>[2x]MKELFQKIWQNELQFLNFDAKFQDKSKLDTAECAIILSVNKDNYERYFLLKEFQELCKKIDLRVDIFSMQNAQICILNLFKSGFISKQDLLKALKILEKISKNTEIFDFILQEKVQSIDQKALFQNDFKELNTINLELQKLSFDENLKSRLQKTLEKFQNLEFNIAITGVMNAGKSSLLNALLKEDFLGVSNIPETANLTVLSYGKSEEAKIYFWDKKEWQNILESSHFNADLKEFIDKLDKSVNIEDFIKDKPLIQNIALCELKNFSSAKNKISALIKKIEIKSHLEFLKNNISIVDTPGLDDVVVQREIVTNEYLRESDFLIHLMNASQSLTQKDADFLVHCLLNSRLSKFLIVLT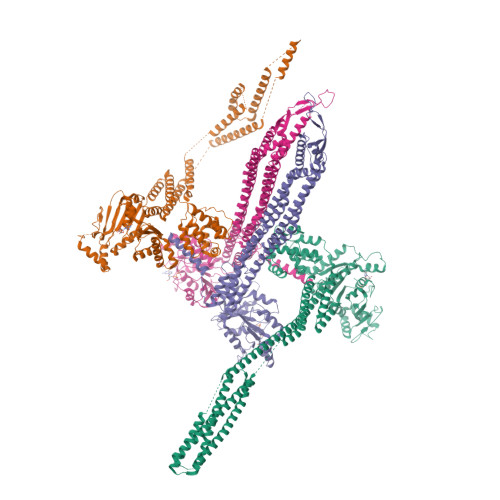KADLLSKKDLEEVIVYTKESLKSRLVDLDENLVEKIDFLCVSAKMASDFYKGLASKESLQKSGMQEFENYLFNELYAGEKSKIALRAYKKELHLELKNILSEYEMQNRLIKENKQGVSEENQKLLLELQKQNTLLKEAQDEISNSIAKLKNIDSGIDNLVLLLAKKLKERLIDEFKYLKNNAQKLNLSRILNIVDITTKDGINDILREIKFENIKKIEELKTNLSLKYDFLKDDFDNGFEGFKDGISKNIDSIFQSEKFALLRLKIEKLSNLKSDLYELETNLDTVIFDTFKEFKMSEILNSLNINGAFFEFLNDKLKHYEKNQKSKLESLEKVLQSLKNQDANILNSFEENLEKIEKLKQLEMGLLNADKLHH;>[2x]GSHMQINLLNDFIKAYENTYSVSFDDSFKGRIQELCKELNEPFMHASYALENELKELVFSLDKNVNIAIIGQFSSGKSSLLNLILGRDCLPTGVVPVTFKPTFLRYAKEYFLRVEFEDGSDIITNIEKLAFYTDQRNEVKQAKSLHIFAPIPLLEKITLVDTPGLNANENDTLTTLDELKNIHGAIWLSLIDNAGKKSEEDAIKANLELLGENSICVLNQKDKLSAEELDNVLNYAKSVFLKYFNELIAISCKEAKDEQSYEKSNFQSLLDFLTQLDTTVLKEKFVKRKILNLCEILEDENQLFVGIFDRLLNQFQSYEKHLLLAYENFLKEIEILNHQILEQLKSISERISSEIFASVKEKDAYFYKESKGFLKKDLYTRYDYKAPYISSDDAFLAMFYNSDVMSKEFKKIKNELYKSFEEIKMKLKDFINILEREILLFKAEFSNIQKDHIFQSDKNFSELRAFCNASDEYFLKDFKELLFKSILELDLFFEKLNLKAFTNYENATKLSLAFFSRKINESRVLYELDSSEFVLFYPKKSEIYERVLNELNVYEFETLLINKPILTKIAKNFLEQSQNLIQEKNKFLDLKKAELQKRRAQILNVRESIKEDHH>PMFIVNTNVPRASVPDGFLSELTQQLAQATGKPPQYIAVHVVPDQLMAFGGSSEPCALCSLHSIGKIGGAQNRSYSKLLCGLLAERLRISPDRVYINYYDMNAANVGW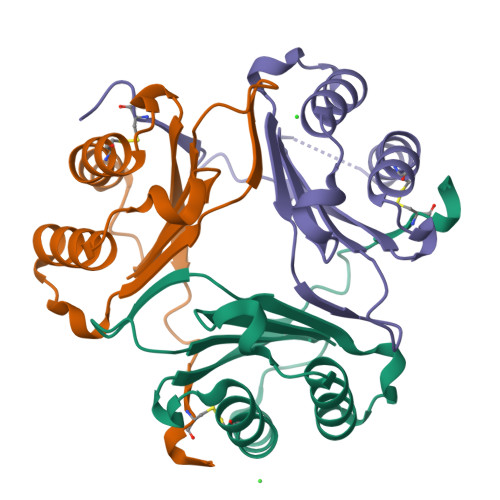NCSTFA[9x]(4S)-1-[(2S,3S,11bS)-2-amino-9,10-dimethoxy-1,3,4,6,7,11b-hexahydro-2H-pyrido[2,1-a]isoquinolin-3-yl]-4-(fluoromethyl)pyrrolidin-2-one | C20 H28 F N3 O3 | 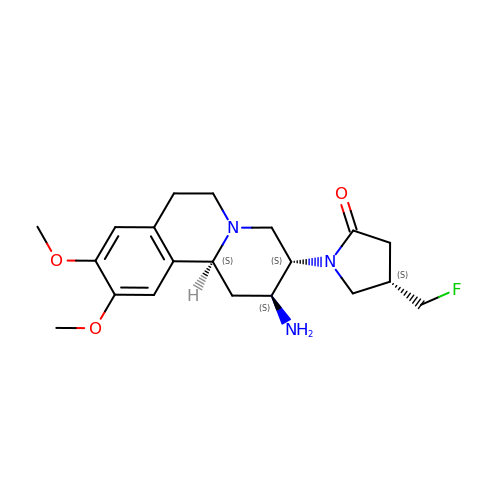GUYMHFIHHOEFOA-ZCPGHIKRSA-N The enzyme CdaA, which synthesizes an essential second messenger cyclic di-AMP (c-di-AMP) in many pathogenic bacteria, has emerged as a promising candidate for the development of novel antibiotics. Additionally, c-di-AMP regulates the bacterial stringent response, further underscoring its significance. The synthesis of c-di-AMP is mediated by enzymes possessing a diadenylate-cyclase (DAC) domain.

Consequently, we selected B. subtilis CdaA for the fragment-screening campaign due to the excellent diffraction properties, high reproducibility and quality of BsCdaA crystals. Notably, these crystals tolerated up to 20% DMSO in the reservoir solution, which facilitates soaking experiments. A crystallographic fragment screen of BsCdaA utilizing the F2X-Entry Screen resulted in a 33% hit rate, identifying 24 distinct fragments interacting with BsCdaA across eight sites.

>[2x]GPTPVEEAQQKTIEAITKAINYMAKRRIGALLTIERDTGMGDYIETGIPLNAKVSSELLINIFIPNTPLHDGAVIMKNNEIAAAACYLPLSESPFISKELGTRHRAAVGISEVTDSLTIIVSEETGGVSVAKNGDLHRELTEEALKEMLEAEFK> MPRLIKERVPTPERSVGERVRDFGEVNLGYSWELALREAERCLQCPVEYAPCIKGCPVHINIPGFIKALRENRDNPSKAVREA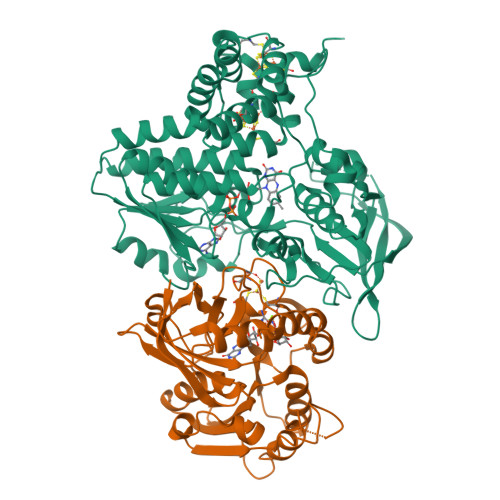LRIIWRDNTLPAITGRVCPQEEQCEGACVVGKVGDPINIGKLERFVADYAREHGIDDELLLEEIKGIKRNGKKVAIIGAGPAGLTCAADLAKMGYEVTIYEALHQPGGVLTYGIPEFRLPKEILRKELKKLSLLGVEIKTDHIVGKTITIQELLQEYDAVFIGTGAGTPKLPNIPGINLNGIYSANEFLTRINLMKAYKFPEYDTPIVVGKKVVVIGAGNTAMDAARSALRLGAEVTIAYRRGREDMTARIEEVKHAEEEGVKFMFFVNPVEFIGDENGNVKAVKFEKMKPLEERDSRGKRKIVGTGEYITVEADTVIIAIGQTPNKVLWRATPELKVDEWGRIVVDENLMTSIPGVFAGGDAIRGEATVILAMGDGRKAAKAIHQYLSKKGN;> MYKILEKKEIAMRNTWYKVYAPHVAKKVQPGQFVIVRAFPNGERIPLTPVMWDREEGWIVLIVFTRGKTTMRMAVELKEGDSLLNVAGPLGTPVPMEKFGKILAIGAYTGIVEVYPIAKAWQEIGNDVTTLHVTFEPMVILKEELEKAVTRHIVEPVPLNPNQDFLANMKNVSQRLKEKVRELLESEDWDLVFMVGPVGDQKQVFEVVKEYGVPMKVDLHPIMVDGTGMCGACRVTVGGEVKFACVDGPEFDAYQVDWDELIHRVGFYAKLEKLALEKYMEELKAKGVI5-(3-{4-[(2S)-2-hydroxy-3,3-dimethylbutoxy]-3-methylphenyl}pentan-3-yl)-3-methyl-N-(1H-tetrazol-5-yl)thiophene-2-carboxamide 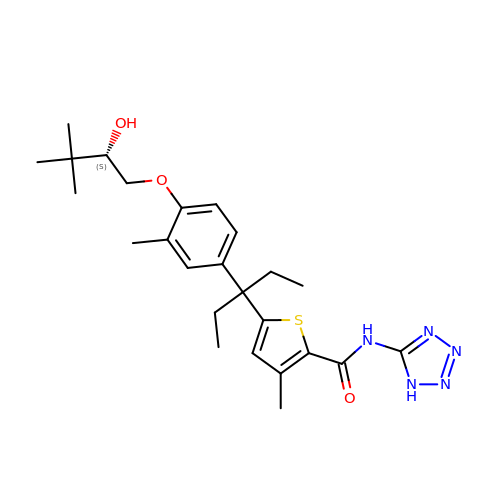| C25 H35 N5 O3 S | XZOVDHKWBOZRPS-LJQANCHMSA-N> MSHSDLTFCEIILMEMESHDAAWPFLEPVNPRLVSGYRRIIKNPMDFSTMRERLLRGGYTSSEEFAADALL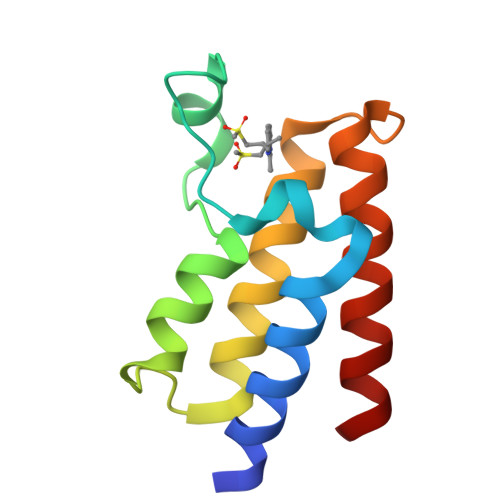VFDNCQTFNEDDSEVGKAGHIMRRFFESRWEEFY> MSNGPEPHGNKIEQPEIRADERQDAGGPANGAPSTSGGAYSQGAKSGGQAAPDPSGSYGIKDAPVAPATIAFEFDGQQVEAQPGETIWAVAKRLGTHIPHLCHKPDPGYRPDGNCRACMVEIEGERVLAASCKRTPAIGMKVKSATERATKARAMVLELLVADQPERATSHDPSSHFWVQADVLDVTESRFPAAERWTSDVSHPAMSVNLDACIQCNLCVRACREVQVNDVIGMAYRAAGSKVVFDFDDPMGGSTCVACGECVQACPTGALMPAAYLDANQTRTVYPDREVKSLCPYCGVGCQVSYKVKDERIVYAEGVNGPANQNRLCVKGRFGFDYVHHPHRLTVPLIRLENVPKDANDQVDPANPWTHFREATWEEALDRAAGGLKAIRDTNGRKALAGFGSAKGSNEEAYLFQKLVRLGFGTNNVDHCTRLCHASS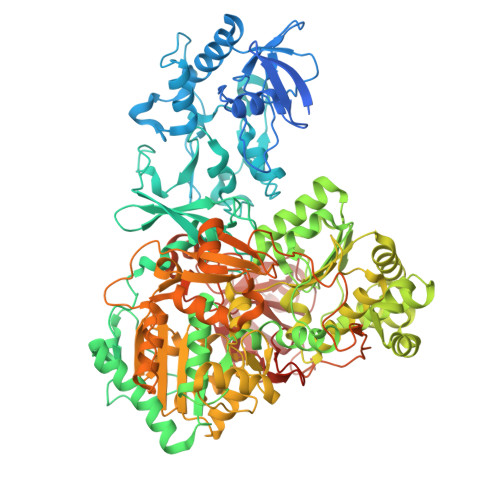VAALMEGLNSGAVTAPFSAALDAEVIVVIGANPTVNHPVAATFLKNAVKQRGAKLIIMDPRRQTLSRHAYRHLAFRPGSDVAMLNAMLNVIVTEGLYDEQYIAGYTENFEALREKIVDFTPEKMASVCGIDAETLREVARLYARAKSSLIFWGMGVSQHVHGTDNSRCLIALALITGQIGRPGTGLHPLRGQNNVQGASDAGLIPMVYPDYQSVEKDAVRELFEEFWGQSLDPQKGLTVVEIMRAIHAGEIRGMFVEGENPAMSDPDLNHARHALAMLDHLVVQDLFLTETAFHADVVLPASAFAEKAGTFTNTDRRVQIAQPVVAPPGDARQDWWIIQELARRLDLDWNYGGPADIFAEMAQVMPSLNNITWERLEREGAVTYPVDAPDQPGNEIIFYAGFPTESGRAKIVPAAIVPPDEVPDDEFPMVLSTGRVLEHWHTGSMTRRAGVLDALEPEAVAFMAPKELYRLGLRPGGSMRLETRRGAVVLKVRSDRDVPIGMIFMPFCYAEAAANLLTNPALDPLGKIPEFKFCAARVVPAEAAPMAAE> MDQSVAESDSNSALEYNKIIGKGVNIGNALEAPFEGAWGVRIEDEYFEIIKKRGFDSVRIPIRWSAHISEKPPYDIDRNFLERVKHVVDRALENNLTVIINTHHFEELYQEPDKYGNVLVEIWRQIAKFFKDYPENLFFEIYNEPAQNLTAEKWNELYPKVLKVIRESNPTRIVIIDAPNWAHYSAVRSLKLVNDKRI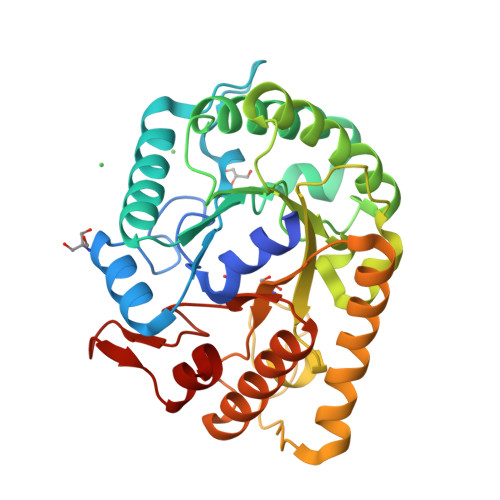IVSFHYYEPFNFTHQGAEWVNPTPPVGVKWNGEEWEINQIRSHFKYVSDWAKQNKVPIFLGEFGAYSKADMDSRVKWTESVRKMAEEFGFSYAYWEFCAGFGIYDRWSQNWIEPLATAVVGESKE>MKLKSFGVFGNPIKHSKSPLIHNACFLTFQKELRFLGHYHPILLPLESHIKSEFLHLGLSGANVTLPFKERAFQVCDKIKGIALECGAVNTLVLENDELVGYNTDALGFYLSLKQKNYQNALILGAGGSAKALACELKKQGLQVSVLNRSSRGLDFFQRLGCDCFMEPPKSAFDLIINATSASLHNELPLNKEVLKGYFKEGKL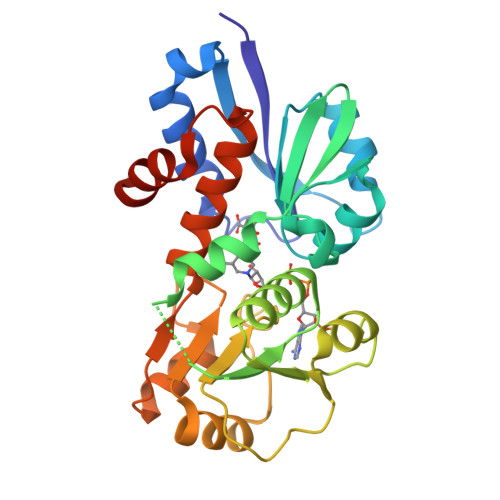AYDLAYGFLTPFLSLAKELKTPFQDGKDMLIYQAALSFEKFSASQIPYSKAFEVMRSVFHHHHHH[2x]> SSDTRKHKFDTSTWALPNKRRRIESEGVGTPSTSPISSLASQKSNCDSDNSITFSRDPFGWNKWKTSAIGSNSENNTSDQKNSYDRRQYGTAFIRKKKVAKQNINNTKLVSRAQSEEVTYLRQIFNGEYKVPKILKEERERQLKLMDMDKEKDTGLKKSIIDLTEKIKTILIENN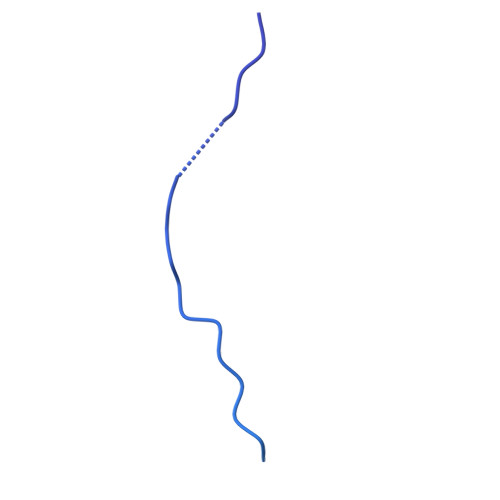KNRLQTRNENDDDLVF>MVKEVVRTDSLKGRRGRLPSKPKSPQEPSPPSPPVSLISALVRAHVDSNPAMTSLDYSRFQANPDYQMSGDDTQHIQQFYDLLTGSMEIIRGWAEKIPGFADLPKADQDLLFESAFLELFVLRLAYRSNPVEGKLIFCNGVVLHRLQCVRGF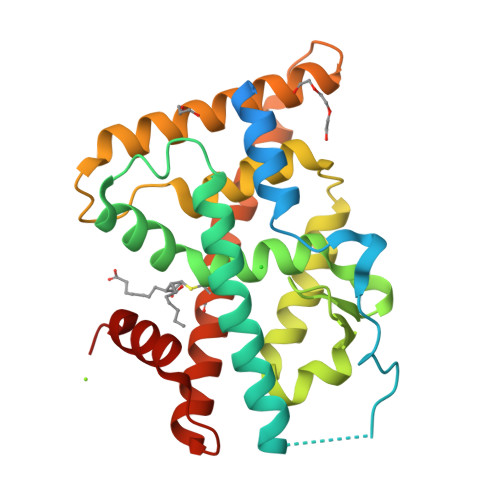GEWIDSIVEFSSNLQNMNIDISAFSCIAALAMVTERHGLKEPKRVEELQNKIVNCLKDHVTFNNGGLNRPNYLSKLLGKLPELRTLCTQGLQRIFYLKLEDLVPPPAIIDKLFLDTLPF[2x]Given the auxotrophic nature of pneumococci for certain amino acids, the Ami ABC transporter system, orchestrating oligopeptide uptake, becomes indispensable in host compartments lacking amino acids. The system comprises five exposed Oligopeptide Binding Proteins (OBPs) and four proteins building the ABC transporter channel. Crucially, SBPs determine the specificity of their respective transport systems, thereby governing the range of molecules capable of entering the cell. The five lipoproteins exhibit pairwise sequence identity of ~52–60% and share a very similar overall folding.

To evaluate AliB’s capacity to recognize diverse peptides, the protein was incubated with an excess of defined synthesized peptides (peptides 2, 3 and 4) that were previously reported to bind AliB. Specifically, crystal structures of AliB in complex with peptide 2 (AIQSEKARKHN), peptide 3 (PIVGGHEGAGV), and peptide 4 (VMVKGPGPGREST) were solved at resolutions of 2.29 Å, 1.66 Å and 1.49 Å, respectively. The three complexes obtained for AliB exhibited minimal backbone changes among them (rmsd ranging between 0.1 and 0.3 Å). In all three complexes, mirroring the observation in the AliD:peptide 1 complex, the amine N-terminus of the oligopeptide establishes a salt-bridge with an aspartic residue (D503) and van der Waals interactions with the neighboring tryptophan residue (W500). The last AliB complex, AliB:peptide 4 (VMVKGPGPGREST), exhibits a recognition pattern akin to the description provided above for the initial three residues of the ligand. Nevertheless, two notable distinctions emerge compared to the previous cases. Firstly, a cis peptide bond is present at position 6 of the peptide, corresponding to a proline. Secondly, the electron density representing the last three peptide residues (EST) weakens significantly, indicating a lack of stabilization for the C-terminus of the ligand. Consequently, the first three positions of the oligopeptides precisely aligned with the AliB binding site, whereas beyond the fourth position, different conformations of the oligopeptide are observed.

> NSSTASKTYNYVYSSDPSSLNYLAENRAATSDIVANLVDGLLENDQYGNIIPSLAEDWTVSQDGLTYTYKLRKDAKWFTSEGEEYAPVTAQDFVTGLQYAADKKSEALYLVQDSVAGLDDYITGKTSDFSTVGVKALDDQTVQYTLVKPELYWNSKTLATILFPVNADFLKSKGDDFGKADPSSILYNGPFLMKALVSKSAIEYKKNPNYWDAKNVFVDDVKLTYYDGSDQESLERNFTAGAYTTARLFPNSSSYEGIKEKYKNNIIYSMQNSTSYFFNFNLDRKSYNYTSKTSDIEKKSTQEAVLNKNFRQAINFAFDRTSYGAQSEGKEGATKILRNLVVPPNFVSIKGKDFGEVVASKMVNYGKEWQGINFADGQDPYYNPEKAKAKFAEAKKELEAKGVQFPIHLDKTVEVTDKVGIQGVSSIKQSIESVLGSDNVVIDIQQLTSDEFDSSGYFAQTAAQKDYDLYHGGWGPDYQDPSTYLDIFNTNSGGFLQNLGLEPGEANDKAKAVGLDVYTQMLEEANKEQDPAKRYEKYADIQAWLIDSSLVLPSVSRGGTPSLRRTVPFAAAYGLTGTKGVESYKYLKVQDKIVTTDEYAKAREKWLKEKEESNKKAQEELAKHVK;> VMVKGPGPGR>[3x]SGKPVLHYFNARGRMECIRFLLAAAGVE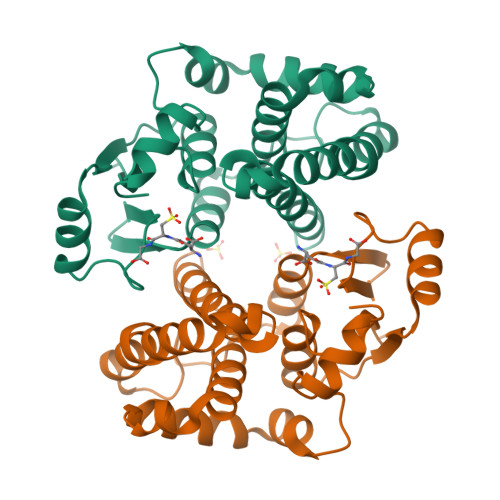FDEKFIQSPEDLEKLKKDGNLMFDQVPMVEIDGMKLAQTRAILNYIATKYDLYGKDMKERALIDMYSEGILDLTEMIMQLVICPPDQKEAKTALAKDRTKNRYLPAFEKVLKSHGQDYLVGNKLTRVDIHLLELLLYVEEFDASLLTSFPLLKAFKSRISSLPNVKKFLQPGSQRKLPMDAKQIEEARKIFKF>[4x]SLPCDICKTVVTEAGNLLKDNATQEEILHYLEKTCEWIHDSSLSASCKEVVDSYLPVILDMIKGEMSNPGEVCSALNLCQSLQ

Saposins are lipid transfer proteins required for the degradation of sphingolipids in the lysosome. These small proteins bind lipids by transitioning from a closed, monomeric state to an open conformation exposing a hydrophobic surface that binds and shields hydrophobic lipid tails from the aqueous environment. Saposins are required for sphingolipid degradation by lysosomal hydrolases; in particular, SapA acts as a co-factor for the enzyme β-galactosylceramidase (GALC) by solubilising its galactosphingolipid substrates. Although individual saposins have low sequence identity (less than 35%), they adopt a common fold consisting of four amphipathic α-helices.

Here we present the crystal structure of a unique tetrameric assembly of murine saposin A produced serendipitously, following modifications of published protocols for making lipoprotein nanodiscs. Four SapA molecules in an open conformation form a diamond-shaped assembly possessing three orthogonal two-fold rotation axes. This symmetry is not perfect as the individual monomers possess small differences in the conformations of loop regions and the C-terminal helix (RMSDs 0.8–1.4 Å over 80 Cα residues), resulting in non-crystallographic symmetry of the tetramer. Each chain of the tetramer interacts directly with the three other chains burying a total surface area of 1210 Å2 for each monomer, representing approximately 20% of the SapA surface. The equivalent dimer within the tetramer structure is very different, possessing a head-to-head arrangement of monomers and substantial direct protein-protein interactions. Comparison of these structures suggests that the tetrameric assembly of SapA is not compatible with binding to GALC without some structural rearrangement. The core of the SapA tetramer structure is hollow and potentially solvent-accessible if it is not filled with amphipathic molecules. Considering the highly hydrophobic nature of the internal SapA surface, exposure of this hollow core to solvent would be thermodynamically unfavourable. It is therefore likely that disordered PC and/or DDM molecules are present in this internal cavity.> QPLLD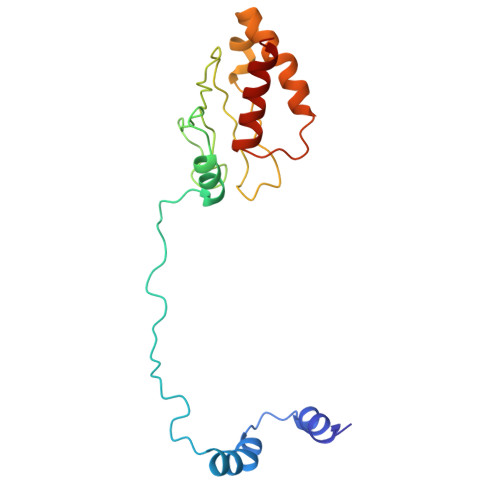AVLANIRSPVFNHSLYRTFVPAMMAIHGPPIVSPVVCSRKRRFEEDERQSIPNVLQGEVARLDPKFLVNLDPSHCSNNGTVHLICKLDDKDLPSVPPLELSVPADYPAQSPMWIDRQWQYDANPFLQSVHRCMTSRLLQLPDKHSVTALLNTWAQSIHQACL>[2x]MSRAYDLVVIGAGSGGLEAGWNAASLHKKRVAVIDLQKHHGPPHYAALGGTCVNVGCV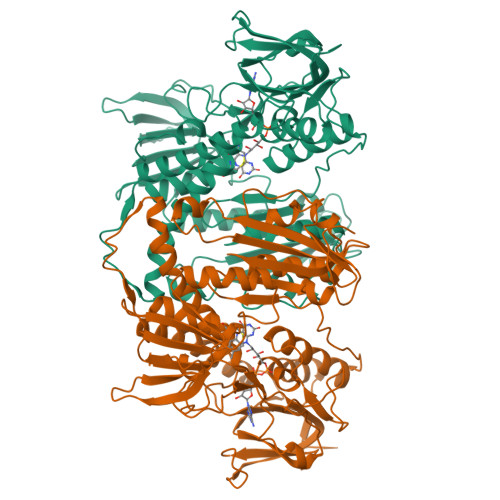PKKLMVTGANYMDTIRESAGFGWELDRESVRPNWKALIAAKNKAVSGINDSYEGMFADTEGLTFHQGFGALQDNHTVLVRESADPNSAVLETLDTEYILLATGSWPQHLGIEGDDLCITSNEAFYLDEAPKRALCVGGGYISIEFAGIFNAYKARGGQVDLAYRGDMILRGFDSELRKQLTEQLRANGINVRTHENPAKVTKNADGTRHVVFESGAEADYDVVMLAIGRVPRSQTLQLDKAGVEVAKNGAIKVDAYSKTNVDNIYAIGDVTDRVMLTPVAINEGAAFVDTVFANKPRATDHTKVACAVFSIPPMGVCGYVEEDAAKKYDQVAVYESSFTPLMHNISGSTYKKFMVRIVTNHADGEVLGVHMLGDSSPEIIQSVAICLKMGAKISDFYNTIGVHPTSAEELCSMRTPAYFYQKGKRVEKI>MSHHHHHHSMASGFIEIANKQGLTATLLPFGATLAKLTFPDKNGKNQDLVLGFDTIDEFEKDAASIGKTVGRVANRIKNSTLHFDGKQYTMTPNNGPHYLHGGPNGLGYRKWEVVRHAPESVSFSVRANEQDDGLPGDAKIDVTYTVNDRNQLIIEHHATCDTPGLLALTNHAYWNLDGSDTVAEHFLEMEADEFVEVDDTFCPTGAIRSVTDTGFDFRSGKQLKESGKDAEELLDLDNDLVITKKTPPSTPSTYLRFWSEKSGIELSITTSYPVIHLYASKFLDCKGKK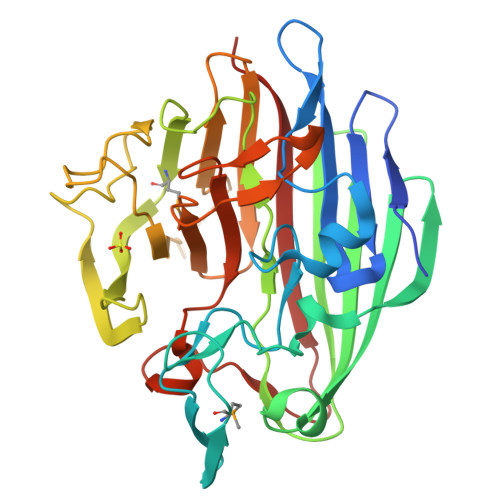GEHYKANKALAIEPQFHSAAPNFDHFPDVSLRPGDHYCQEIVYTFSHVN[2x]Adenosine Deaminases Acting on RNA (ADARs) are members of a family of RNA editing enzymes that catalyze the conversion of adenosine into inosine in double-stranded RNA (dsRNA). Critical in the mechanism of the ADAR reaction, a loop in the protein (i.e., the base-flipping loop) approaches the site of reaction on the dsRNA from the minor groove and the side chain of a glutamic acid (Glu488) present on this loop flips the targeted A into the active site and fills the vacated space. Substrate RNAs with 5′-U are well accommodated while the 2-amino group on 5′-G clashes with Gly489, adjacent to Glu488 of the ADAR2 flipping loop. We identify additional nucleoside analogs that accomplish this in vitro and in cellulo and report a proposed mechanism of action for these analogs based on crystal structures of a truncated homodimer of human ADAR2 bound to dsRNA substrates containing 2′-deoxyinosine or a base-expanded cytidine analog (dyC) paired to the 5′-G.

However, since dI bears a single hydrogen bond donor on its Watson–Crick face, it must engage the 5′-G in a different manner than seen with 3-deaza dA. X-ray crystallography was used to resolve the structure of the ADAR2-R2D E488Q protein bound to an RNA duplex containing a target sequence derived from human glioma-associated oncogene 1 (hGLI1) and a guide oligonucleotide that forms a dI/G pair adjacent to the editing site. To trap the RNA/protein complex for crystallization, we synthesized a duplex substrate containing 8-azaN at the editing site. We were able to grow crystals of the protein/RNA complex that diffracted X-rays to 2.8 Å. The dI/G pair adjacent to the edit site is well defined and shows the 5′-G in the syn conformation with its Hoogsteen face accepting hydrogen bond donation from the protonated N1 of dI. The interaction appears to involve a bifurcated hydrogen bond with N1 of dI donating a strong hydrogen bond to N7 of 5′-G and a slightly weaker hydrogen bond to O6. Superimposition of the dI/G pair observed here with the previously published 3-deaza dA/G pair indicates that due to the bifurcated hydrogen bond, dI shifts in the direction of the major groove and away from the Gly489 position relative to the position of 3-deaza dA. In addition, superimposition of the dI/G pair with the G/G pair clearly shows the benefit of removing the −1 G 2-amino in the minor groove in creating space for the flipping loop. We hypothesize that despite the favorable structural benefits offered by dI at the −1 position, bifurcation of one hydrogen bond may be less stabilizing to the syn:anti pair than the two hydrogen bonds present in the deaza-dA/G substrates. This may explain the lower in vitro deamination rates on substrates containing a −1 dI.

>[2x]ASLAQPPLPVLPPFPPPSGKNPVMILNELRPGLKYDFLSESGESHAKSFVMSVVVDGQFFEGSGRNKKLAKARAAQSALAAIFNLHLDQTPSRQPIPSEGLQLHLPQVLADAVSRLVLGKFGDLTDNFSSPHARRKVLAGVVMTTGTDVKDAKVISVSTGTKCINGEYMSDRGLALNDCHAEIISRRSLLRFLYTQLELYLNNKDDQKRSIFQKSERGGFRLKENVQFHLYISTSPCGDARIFSPHEPILEEPADRHPNRKARGQLRTKIESGQGTIPVRSNASIQTWDGVLQGERLLTMSCSDKIARWNVVGIQGSLLSIFVEPIYFSSIILGSLYHGDHLSRAMYQRISNIEDLPPLYTLNKPLLSGISNAEARQPGKAPNFSVNWTVGDSAIEVINATTGKDELGRASRLCKHALYCRWMRVHGKVPSHLLRSKITKPNVYHESKLAAKEYQAAKARLFTAFIKAGLGAWVEKPTEQDQFSLTP>MGSDKIHHHHHHMVSRRISEIPISKTMELDAKAKALIKKGEDVINLTAGEPDFPTPEPVVEEAVRFLQKGEVKYTDPRGIYELREGIAKRIGERYKKDISPDQVVVTNGAKQALFNAFMALLDPGDEVIVFSPVWVSYIPQIILAGGTVNVVETFMSKNFQPSLEEVEGLLVGKTKAVLINSPNNPTGVVYRREFLEGLVRLAKKRNFYIISDEVYDSLVYTDEFTSILDVSEGFDRIVYINGFSKSHSMTGWRVGYLISSEKVATAVSKIQSHTTSCINTVAQYAALKALEVDNSYMVQTFKERKNFVVERLKKMGVKFVEPEGAFYLFFKVRGDDVKFCERLLEEKKVALVPGSAF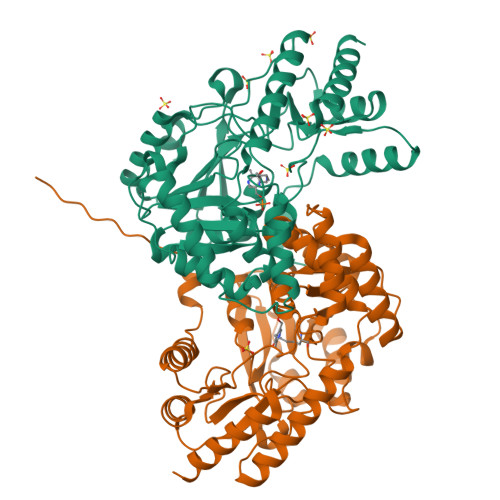LKPGFVRLSFATSIERLTEALDRIEDFLNSR[2x]> SGSGKPAYQIYMEFFQNKQDDHDPIDTFVIQKRALLAQL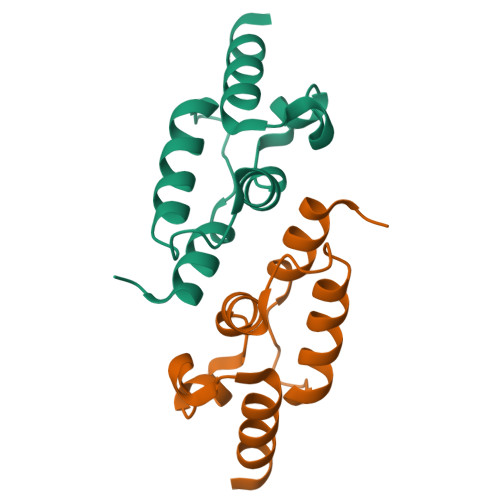PSGRHDEETELDLLFGLLNIKYRKHISRHSVHTFKDLLEQGRIIEHNNQED4-[2-(4,4-dimethyl-1-propan-2-yl-quinolin-6-yl)ethynyl]benzoic acid | 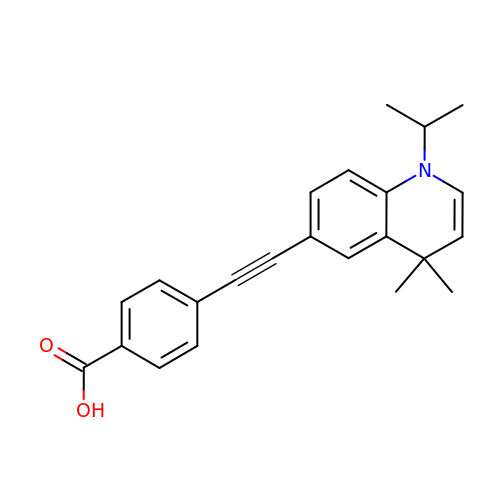C23 H23 N O2 | HXWVRWZLWIKKOS-UHFFFAOYSA-N>ALSAEGSSGGSRGGSPKAEAASVPSWPQILGRLTDNRDLARGQAAWAMDQIMTGNARPAQIAAFAVAMTMKAPTADEVGELAGVMLSHAHPLPADTVPDDAVDVVGTGGDGVNTVNLSTMAAIVVAAAGVPVVKHGNRAASSLSGGADTLEALGVRIDLGPDLVARSLAEVGIGFCFAPRFHPSYRHAAAVRREIGVPTVFNLLGPLTNPARPRAGLIGCAFADLAE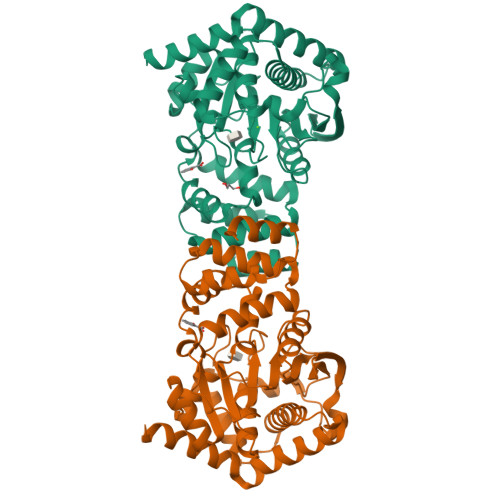VMAGVFAARRSSVLVVHGDDGLDELTTTTTSTIWRVAAGSVDKLTFDPAGFGFARAQLDQLAGGDAQANAAAVRAVLGGARGPVRDAVVLNAAGAIVAHAGLSSRAEWLPAWEEGLRRASAAIDTGAAEQLLARWVRFGRQILEHHHHHH[4x]> 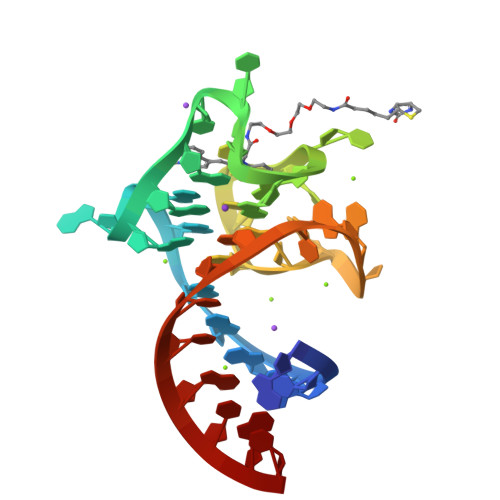GUACGAAGGAAGGUUUGGUAUGGGGUAGUUGUCGUAC> GPLGSMSSMNPEYDYLFKLLLIGDSGVGKSCLLLRFADDTYTESYISTIGVDFKIRTIELDGKTIKLQIWDTAGQERFRTITSSYYRGAHGIIVVYDVTDQESFNNVKQWLQEIDRYASENVNKLLVGNK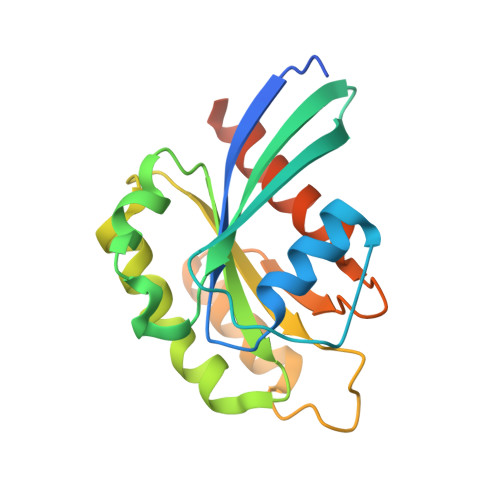CDLTTKKVVDYTTAKEFADSLGIPFLETSAKNATNVEQSFMTMAAEIKKRMGPGATAGGAEKSNVK>ACGSIVPRREWRALASECRERLTRPVRYVVVSHTAGSHCDTPASCAQQAQNVQSYHVRNLGWCDVGYNFLIGEDGLVYEGRGWNIKGAHAGPTWNPISIGISFMG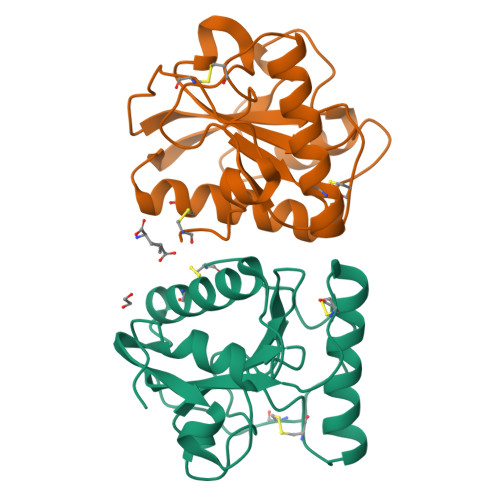NYMNRVPPPRALRAAQNLLACGVALGALRSNYEVKGHRDVQPTLSPGDRLYEIIQTWSHYRA[4x]>[2x]PQFSLWRRPVVTAHIEGQPVEVLLDTGA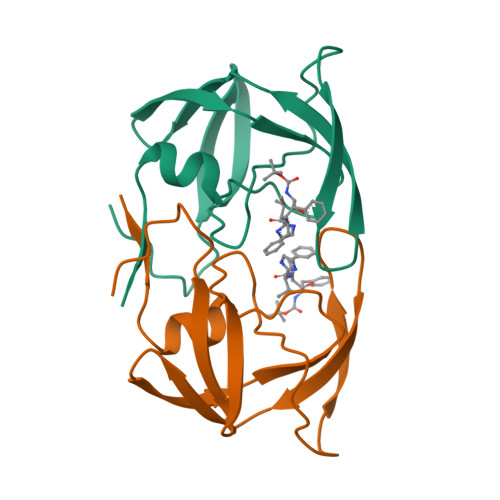DDSIVTGIELGPHYTPKIVGGIGGFINTKEYKNVKIEVLGKRIKGTIMTGDTPINIFGRNLLTALGMSLNL> GSHMASMKKKGSVVIVGRINLSGDTAYAQQTRGEEGCQETSQTGRDKN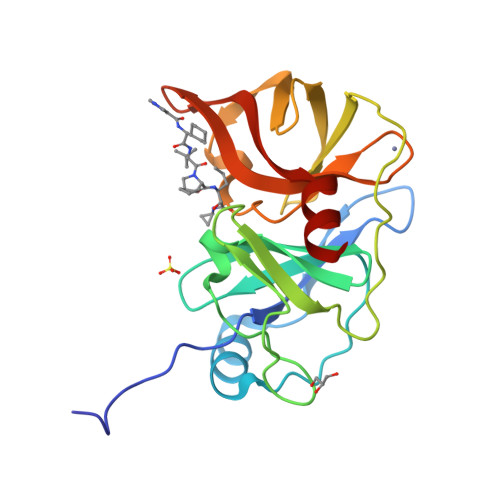QVEGEVQIVSTATQTFLATSINGVLWTVYHGAGTRTIASPKGPVTQMYTNVDKDLVGWQAPQGSRSLTPCTCGSSDLYLVTRHADVIPVRRRGDSRGSLLSPRPISYLKGSSGGPLLCPAGHAVGIFRTAVSTRGVAKAVDFIPVESLETTMRSP>[2x]MPQTAGPDTIRILVSTDNHVGYEERDPIRKDDSWRTFDEIMQLARTKDVDMVLLGGDLFHDNKPSRKAMYQVMRSLRKNCLGMKPCELEFLSDPAEVFEGAFPHVNYYDPDINVSIPVFSIHGNHDDPSGDGHLCSLDLLQVAGLVNYFGRVPEADNIHVKPILLQKGKTKLALYGMSNVRDERIHRTFRDNKVRFYRPSQQTGDWFNLLTLHQNHYAHTPTGYLSENMLPDFLDLVIWGHEHECLIDPKKNPETGFHVMQPGSSIATSLVPGEAVPKHIAILSITGKSFEVEKIPLRTVRPFVIREITLATDKRFKGLEKKQDNRQEVTKRLMQIVEEMIAEANEMWRSLHEDSQDDEDEEQPLPLIRLKVEYSSPEGTKFEVENPQRFSNRFAGKVANQNDVVHFYRKKTGTTRKPKEGKRELPEGIAEALEDSDSISVDALVQEFFAQQSLKILPQAPFGDAVNQFVSKDDKHAVEMFVMDSLSSQVRGLLQLDDDKINEGLDSHIEDFRKVMEKNFLSGQQKQAQRRRRFKEKPEGWDSDLNGHWTLQPEAIEELSSSPEPAKEGGRVRPASRITVGDEDNLFEEEEFVQKTTAKRAPTTRATRKTAAATRATTATKASAPAKKSIAAPRGRKRANPFQDSAEEEEDVIMDDDDDYKPAPPVKAPPPKPARETQTRGAPKTRQTTLNFSQAERPTRTTQKAIEISDDEISEDDAFESMPARKSKRY;>[2x]MSKIEKLSILGVRSFGPHHPETIAFNTPLTLIVGYNGSGKTTVIECLKYATTGELPPNSTRNGAFIHDPDLVGEKEVRAQVKLSFRSTIGESYVVTRNIQLLVQRNNKRTQKTLEGSLLLRNNGERTVISTRVAELDKLVSEKLGVPPAILDAVIFCHQDDSLWPMSEPAALKKRFDEIFEAQKYTKVIENIRLLKKKKGDELKILKEREVQDKANKERAEKVDRLMAQLTREILEAREKCNELSKQMEEESAKIKDKYEQANSFLKIMNDLQTKTEKLEYKKDAIVELRSRIEELPDPDEVLRNTLDEYEQTINRIVADRDHKAAQFHDLQAELKSARDQHTAKAAEQGKHQSDKEKYERQLVARERMIREAAERHEIRGYNGDLDDRRIAIFNERIQKILNDKRRELERLQRENQEELDRKTAVIAERESRKQSVIRDRKAAKDRIISLGKDMASIQGELSSIDIDEGTEEMLRAEMKELQARIEAAKADEQNANLDAQIKEVNEEIWKLESLSAKLARELVECTRLASERAQLDLRRKQLAERKRELEIMTNTWNEQFSTLLGEGWRPETLERDFSDVLKQQQLLVGEHRKKKDATQQELKQAEYQLSNARNLHNKLTNEMEACMRAVQTAMKEARDLDSAPPVDEYITMLETDEKELAEVETALKLYDELKKHYSTIKDRALRFNKCYICDRDFTNQEAAKTRLLEKVAKRLGDEEKKELLEDQAAFMKSLDILRAVRVKYDTYQRLSSELPQLSREIDSETNRREDLVRRLEDQDLAFREADNKLQEMETLNKHVMKITQLLKDISDAEKQVERSQQLSNIETRSADEINEEQTTCAEQT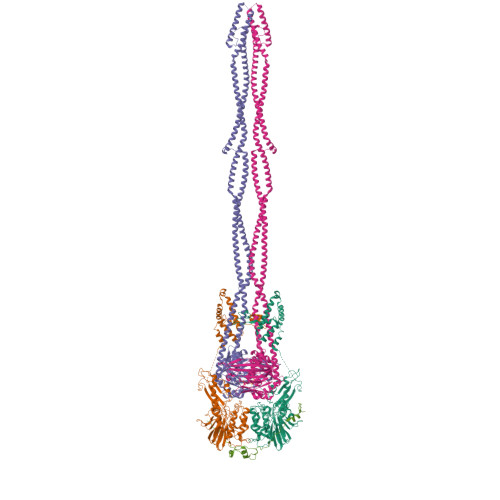RAAQAKLTKLTAEKQRLKDLVRQLEVERLQLENKISSAVQQLERKKRLQESIARHKEDQNQARNAVQEADEELERLEPEIAGARAALDEARQACRAKEQKVAAERDAIAQTVSELNMINSEIQEYLDRGGPSSLAANQRAIANLETQMANLEGEMRELTVQINKLNKEIDNSDAKKRNIADNLTYRKNLREKDALEREIAELEARNAQEDYDRLIKEAHYLEAHRSKLNADRERLMGMMSTKDEEFRRLNEEYELDLKDAKAKYKETHIKVETTKAAIEDLGRGMAAVDHAIMQYHSKMMEQINRTIAELWQSTYQGTDIDTIQIRSDVESTTSSDSGTRRNYNYRVSMVKGDTEMDMRGRCSAGQKVLASIIIRLALAESFCANCGLIALDEPTTNLDSDNIRSLAESLHGIIKARQAQGNLQLIVITHDEEFLKYMQCSDFCDDFYRVKRDEKQNSVIVRESITRITE;> MWILESELFDGKRLWLRPGKTYLFGRTVAEAGQLTISDKTVSRKHLTIHIDNVPEGGGRNLRSRSNVIVEDLESKKGTLVNGVQIRGQKTTLTEDVNEIKLGLCPKTLKIRWHPIVLSFSFTSKELRADPWTNLRDSLEQLDIKYSAEYEPTTTHVVSKKRNTSKGLQALINGRYIVTDSFINAIVQATEIPEGEEGASSALEQDFEANWPNPLDHLPPRGEEPGNHTTETYAPDARRQEVFDGYTFIFYEKKQYDNLFPAISAGKGKALLKEVVPNRTRVDEFVRYVKSVAGEKGLGSFEDGSEGKGVVVVRYTPKGEDSAWYAEFFTKFAQQLDHRPIDQKEFLEAILACDASMLRRPLEAMSQPVSVSASVEPQSSEKVRPAVEDRKEVEQSAPKQLQPSAEVPATEESAPAPHRRERRTGRSRFKGFDFDDDDIIIETPQAQSSTQVPALPQVPSASQDSLFVSQREPSLAPSEPMLEEEAPCNTRTTRQTHRKRVLSPLPEHDNSALLDEIAPITAAVKRRRIEAGQDPVPPLPEPEPEREDEDVEMVEESPPRKGKKGAATTAKGKGKKIKQEDEENVLELARRRREEAEAAAAAERQRLAQLGDDDIDYAAIRRLHIIEEIEVRQPEPHGPNRTREQDIADGRWDPRWNGRKNFKRFRRQGETGVRMPVQSVIVPLEEVRTKEYGIGDDYWLEDEEGRVPRRPKETQTQERSTIGSVRDGSGFAAAAASGKGKEKDKENEKEVGRPGSSAAAAKQRSKPAPRRTVLTLDSSDEDEDEPSPHAPGIDTISDSEPEVVSSFPSVIPASEPSRSRAAKAAERANALRSSAHSSQSQTQQHRESQLSTGSSKIQLTLAPGSSSLSFSRSGTAAGRNENGKRPFGSFVSGESTASGRGMSVESGSVRGESASKRQKQGSSGGGSFLATRRKDDGSEEESEDDELKFRFGRRR>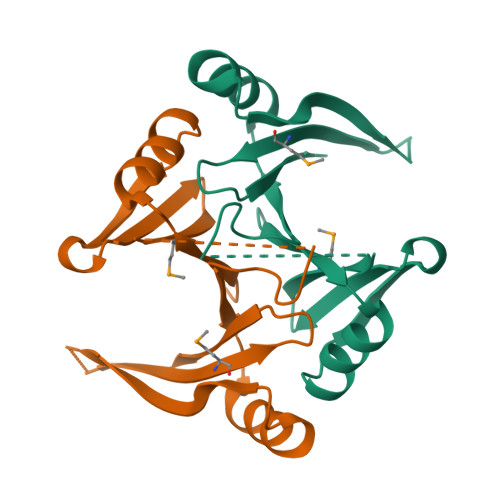[2x]MSLTLRVVPELYCFDINVSQSFFVDVLGFEVKYERPDEEFVYLTLDGVDVMLEGIAGKSRKWLSGDLEFPLGSGVNFQWDVIDIEPLYQRVNESAADSIYLALESKSYQCGDSIATQKQFMVQTPDGYLFRFCQDIHEGHHHHHH> MVSVGDAAFRQEANKKFKYSVKLSDYSTLQDAVTDAVDGLLIDINYNFTDGESVDFXGKILTINCKAKFIGDGALIFNNMGPGSVINQPFMESKTTPWVIFPWDADGKWITDAALVAATLKQSKIEGYQPGVNDWVKFPGLEALLPQNVKDQHIAATLDIRSASRVEIRNAGGLMAAYLFRSCHHCKVIDSDSIIGGKDGIITFENLSGDWGLGNYVIGGRVHYGSGSGVQFLRNNGGESHNGGVIGVTSWRAGESGFKTYQGSVGGGTARNYNLQFRDSVALSPVWDGFDLGSDPGMAPEPDRPGDLPVSEYPFHQLPNNHLVDNILVMNSLGVGLGMDGSGGYVSNVTVQDCAGAGMLAHTYNRVFSNITVIDCNYLNFDSDQIIIIGDCIVNGIRAAGIKPQPSNGLVISAPNSTISGLVGNVPPDKILVGNLLDPVLGQSRVIGFNSDTAELAL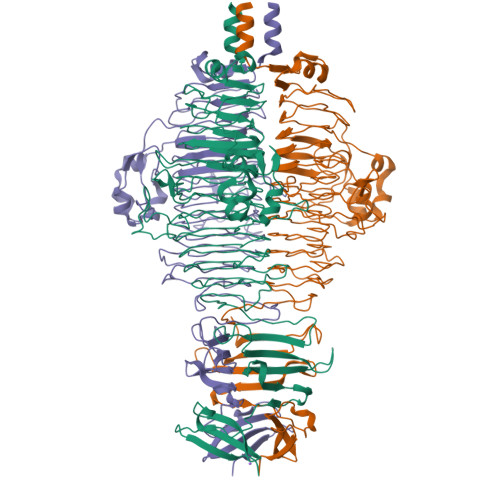RINKLSATLDSGALRSHLNGYAGSGSAWTELTALSGSTPNAVSLKVNRGDYKTTEIPISGTVLPDEGVLDINTMSLYLDAGALWALIRLPDGSKTRMKLSV>[3x]MTKRVRLSDSFNPVYPYEDESTSQHPFINPGFISPNGFTQSPNGVLTLKCLTPLTTTGGSLQLKVGGGLTVDDTNGFLKENISATTPLVKTGHSIGLPLGAGLGTNENKLCIKLGQGLTFNSNNICIDDNINTLWTGVNPTEANCQIMNSSESNDCKLILTLVKTGALVTAFVYVIGVSNNFNMLTTHRNINFTAELFFDSTGNLLTRLSSLKTPLNHKSGQNMATGAITNAKGFMPSTTAYPFNDNSREKENYIYGTCYYTASDRTAFPIDISVMLNRRAINDETSYCIRITWSWNTGDAPEVQTSATTLVTSPFTFYYIREDD;>MARSPGRAYALLLLLICFNVGSGLHLQVLSTRNENKLLPKHPHLVRQKRAWITAPVALREGEDLSKKNPIAKIHSDLAEERGLKITYKYTGKGITEPPFGIFVFNKDTGELNVTSILDREETPFFLLTGYALDARGNNVEKPLELRIKVLDINDNEPVFTQDVFVGSVEELSAAHTLVMKINATDADEPNTLNSKISYRIVSLEPAYPPVFYLNKDTGEIYTTSVTLDREEHSSYTLTVEARDGNGEVTDKPVKQAQVQIRILDVNDNIPVVENKVLEGMVEENQVNVEVTRIKVFDADEIGSDNWLANFTFASGNEGGYFHIETDAQTNEGIVTLIKEVDYEEMKNLDFSVIVANKAAFHKSIRSKYKPTPIPIKVKVKNVKEGIHFKSSVISIYVSESMDRSSKGQIIGNFQAFDEDTGLPAHARYVKLEDRDNWISVDSVTSEIKLAKLPDFESRYVQNGTYTVKIVAISEDYPRKTITGTVLINVEDINDNCPTLIEPVQTICHDAEYVNVTAEDLDGHPNSGPFSFSVIDKPPGMAEKWKIARQESTSVLLQQSEKKLGRSEIQFLISDNQGFSCPEKQVLTLTVCECLHGSGCREAQHDSYVGLGPAAIALMILAFLLLLLVPLLLLMCHCGKGAKGFTPIPGTIEMLHPWNNEGAPPEDKVVPSFLPVDQGGSLVGRNGVGGMAKEATMKGSSSASIVKGQHEMSEMDGRWEEHRSLLSGRATQFTGATGAIMTTETTKTARATGASRDMAGAQAAAVALNEEFLRNYFTDKAASYTEEDENHTAKDCLLVYSQEETESLNASIGCCSFIEGELDDRFLDDLGLKFKTLAEVCLGQKIDINKEIEQRQKPATETSMNTASHSLCEQTMVNSENTYSSGSSFPVPKSLQEANAEKVTQEIVTERSVSSRQAQKVATPLPDPMASRNVIATETSYVTGSTMPPTTVILGPSQPQSLIVTERVYAPASTLVDQPYANEGTVVVTERVIQPHGGGSNPLEGTQHLQDVPYVMVRERESFLAPSSGVQPTLAMPNIAVGQNVTVTERVLAPASTLQSSYQIPTENSMTARNTTVSGAGVPGPLPDFGLEESGHSNSTITTSSTRVTKHSTVQHSYS[2x]

Among human species B adenovirus, HAdV-11, has the particular feature of exploiting two primary receptors, desmoglein 2 (DSG2) and CD46, to mediate cell attachment. Interactions between HAdV-11 and CD46 are well-characterized and clearly depend on the fiber protein, but the mechanism whereby HAdV-11 engages DSG2 has been still unresolved. In this study, we elucidate the molecular basis for HAdV-11 recognition of DSG2 by resolving the structure of extracellular domains of DSG2 in complex with the HAdV-11 fiber knob protein. The structure shows that DSG2 and CD46 engage different HAdV-11 residues and interfaces without overlapping.

During the image analysis, two main populations of particles consisting of the HAd11K in complex with either one or two rDSG2 modules were identified and two 3D reconstructions were obtained at 3.5 and 3.2 Å resolution for HAd11K in complex with one or two rDSG2, respectively. The binding of rDSG2 to HAd11K is very similar in both populations meaning that the binding of a second rDSG2 is possible without interfering with the first rDSG2. Moreover, in the population with two rDSG2 attached to the HAd11K, each rDSG2 binds HAd11K in the same way with the same interfacing residues. rDSG2 consists of two modules, EC2 and EC3, and each one interacts with a different monomer of HAd11K. The tips of two loops in EC2 (around residue A125 and residues S175, T177, respectively) are in close contact with residues located on the apex of the HAd11K (in particular residues N190 and N192). Several putative hydrogen bonds are predicted in this region which likely contributes to the binding. Regarding the interaction of the EC3 module of rDSG2 with HAd11K, the loop region centered around R316 of EC3 fits snugly in an apical region of HAd11K defined by two loops centered around D265 and D300, respectively. Several hydrogen bonds and salt bridges are also predicted in this area. The interacting regions of rDSG2 on HAd11K are strikingly similar to the one found for HAd7K and HAd3K, two other adenoviruses which are using DSG2 as their cellular receptor. Indeed, HAd11K and HAd7K are very similar in sequence (92.9% identity), and the interacting residues with rDSG2 are very well conserved at the exception of the D300 in HAd11K which is replaced by V300 in HAd7K. As reported for the other two serotypes, −3 and −7, the structure shows that EC2 and EC3 ectodomains bind at the top of the trimeric knob and that D265 mediates central contacts with DSG2 (19, 21).>LAKLYKVSNGAGTMSVSLVADENPFAQGALKSEDCFILDHGKDGKIFVWKGKQANTEERKAALKTASDFITKMD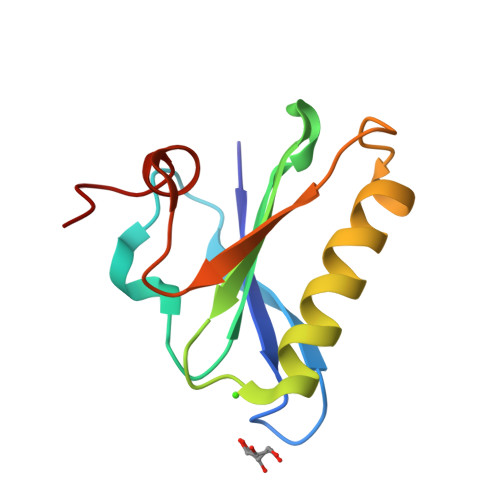YPKQTQVSVLPEGGETPLFKQFFKNWR[2x]>GSHMWDTANNPLYKE[2x];>PVQLNLLYVQARDDILNGSHPVSFDKACEFAGYQCQIQFGPHNEQKHKPGFLELKDFLPKEYIKQKGERKIFMAHKNCGNMSEIEAKVRYVKLARSLKTYGVSFFLVKEKMKGKNKLVPRLLGITK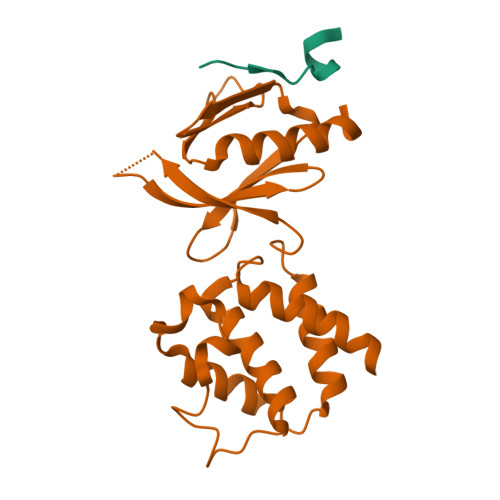ECVMRVDEKTKEVIQEWSLTNIKRWAASPKSFTLDFGDYQDGYYSVQTTEGEQIAQLIAGYIDIIL[2x]~{N}-[4-[5-(3-aminophenyl)-6-(1-methylpyrazol-4-yl)furo[2,3-d]pyrimidin-4-yl]oxyphenyl]-2-(4-fluorophenyl)-1-methyl-3-oxidanylidene-pyrazole-4-carboxamide 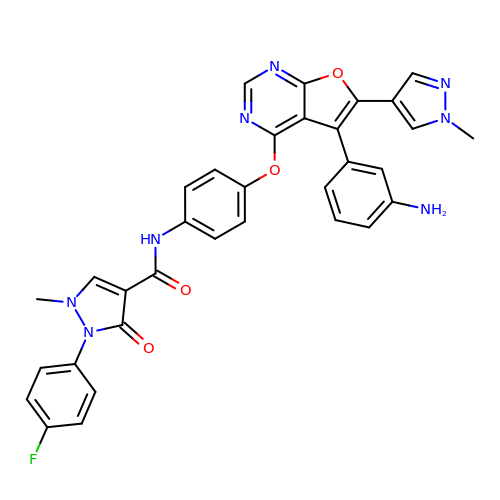| C33 H25 F N8 O4 | ROQFVBHLGRGANE-UHFFFAOYSA-N Laccases are four-copper oxidases that catalyze the oxidation of phenolic units in lignin as well as a wide range of phenolic compounds and aromatic amines. Because of their oxidoreductase activity, laccases can react with 2,2′-azino-bis(3-ethylbenzothiazoline-6-sulphonic acid) (ABTS) as a substrate and as a mediator for studying laccase-mediator systems. In addition, our previously discovered Cerrena sp. RSD1 laccase, DLac, had the highest organic-solvent enhancement and tolerance among the fungal laccases tested. We found that pre-incubation of fungal laccases with certain organic solvents significantly increased their activity toward both phenolic and non-phenolic substrates.

We also crystalized acetone-pre-incubated DLac to investigate whether the protein was modified or bonded by acetone molecules. DLac after 1-day acetone-pre-incubation was prepared for crystallization. At the crystallization stage, the crystal-growth time was 2, 9 and 20 days with pre-incubated acetone concentration 30%, 20% and 0%, respectively, which suggests that acetone may accelerate DLac crystallization. The space group was changed to P43212, different from the orthorhombic form of P212121. However, this tetragonal crystal structure showed neither binding of the acetone molecule nor any chemical modification. Two crystal structures could be perfectly superimposed with an overall RMSD of 0.143 Å for 494 C atoms. Notably, CD and crystal structure analysis indicated that even at high acetone concentration, the 3-D structure of DLac was not damaged. Thus, this immediately reversible enhancement was due to neither chemical modification nor covalent binding with solvent molecules. Here, DLac, with a broader substrate-binding cavity, showed higher organic-solvent enhancement than TvLac (3-fold vs 1.5-fold).

> AVGPVTDIHIVNKDIAPDGFSRPSVLAGGTFPGPLITGQKGDNFKLNVVDDLTDASMLKSTSIHWHGFFQKGTNWADGPAFVNQCPISTGNSFLYNFQVPDQAGTYWYHSHLSTQYCDGLRGAFVVYDPTDPHKALYDVDDESTVITLADWYHTLARQIVGVAIADTTLINGLGRNTNGPADAALAVINVEAGKRYRLRLVSISCDPNYVFSIDNHDFNIIEVDGVNSKPLNVDSIQIFAGQRYSAVLNANQPVGNYWVRANPNLGTTGFTGGINSAILRYKGAPVAEPTTTQTTSTKPLQEPNLRPLVSMPVPGSATPGGVDVVHNLILGFSAGKFTINGAAFTPPSVPVLLQILSGTTNAQDLLPSGSVITLPIGKTIELTLAAGVLGGPHPFHLHGHNFHVVRSAGQTTPNYVDPIVRDVVNTGGTGDNVTIRFTTDNPGPWFLHCHIDWHLEAGFAVVFAEGVNQTNAANPTPADWNNLCNIYNALADGDK> RRRRRRRRR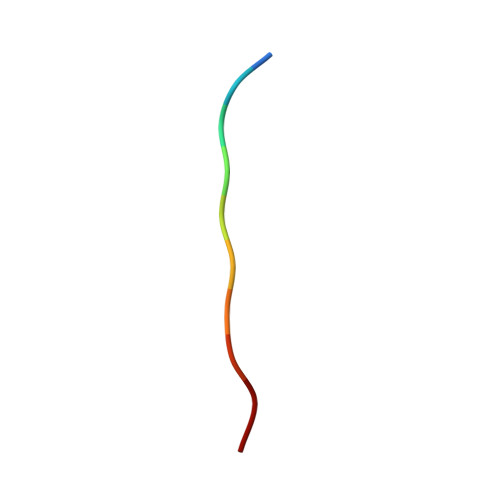R> MENTENSVD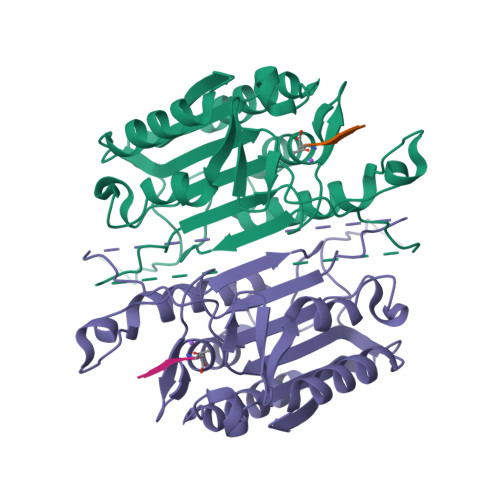SKSIKNLEPKIIHGSESMDSGISLDNSYKMDYPEMGLCIIINNKNFHKSTGMTSRSGTDVDAANLRETFRNLKYEVRNKNDLTREEIVELMRDVSKEDHSKRSSFVCVLLSHGEEGIIFGTNGPVDLKKITNFFRGDRCRSLTGKPKLFIIQACRGTELDCGIETDSGVDDDMACHKIPVEADFLYAYSTAPGYYSWRNSKDGSWFIQSLCAMLKQYADKLEFMHILTRVNRKVATEFESFSFDATFHAKKQIPCISSMLTKELYFYHL>[2x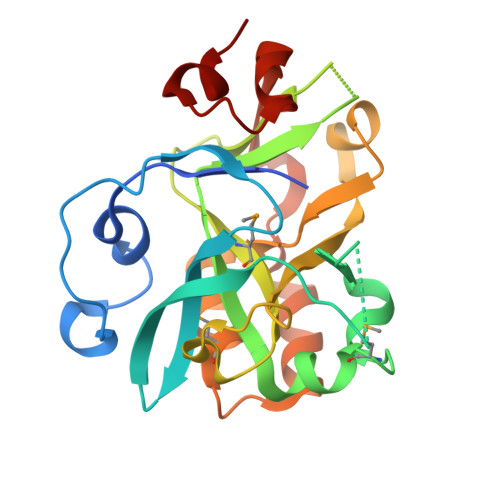]GSSGSSGMCGRFAQSQTREDYLALLAEDIERDIPYDPEPIGRYNVAPGTKVLLLSERDEHLHLDPVFWGYAPGWWDKPPLINARVETAATSRMFKPLWQHGRAICFADGWFEWKKEGDKKQPFFIYRADGQPIFMAAIGSTPFERGDEAEGFLIVTAAADQGLVDIHDRRPLVLSPEAAREWMRQEISGKEASEIAASGCVPANQFSWHPVSRAVGNVKNQGAELIQPV methyl 2-acetamido-4-O-{2-acetamido-4,6-O-[(1S)-1-carboxyethylidene]-2-deoxy-beta-D-mannopyranosyl}-2-deoxy-beta-D-glucopyranoside | C20 H32 N2 O13 | 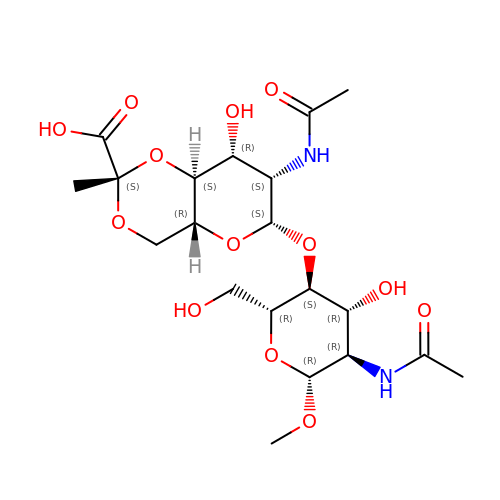UVHDIWJHCZODAO-MYXXRMNRSA-N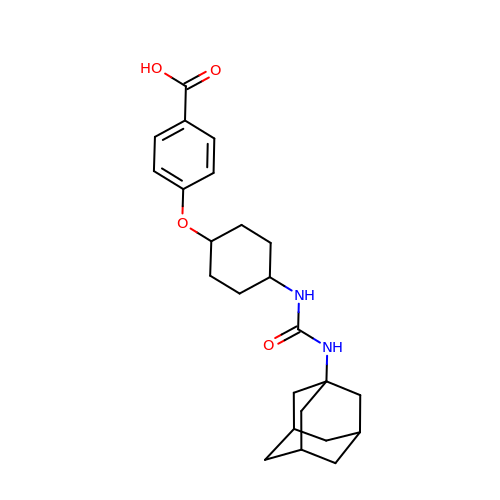4-[(trans-4-{[(3s,5s,7s)-tricyclo[3.3.1.1~3,7~]dec-1-ylcarbamoyl]amino}cyclohexyl)oxy]benzoic acid | C24 H32 N2 O4 | KNBWKJBQDAQARU-GNCKNZPZSA-N> VEDYEQG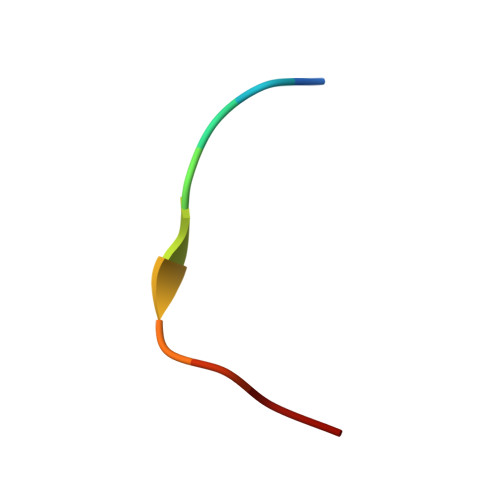LSG> GSHMASMKKKGSVVIVGRINLSGDTAYAQQTRGEEGCQETSQTGRDKN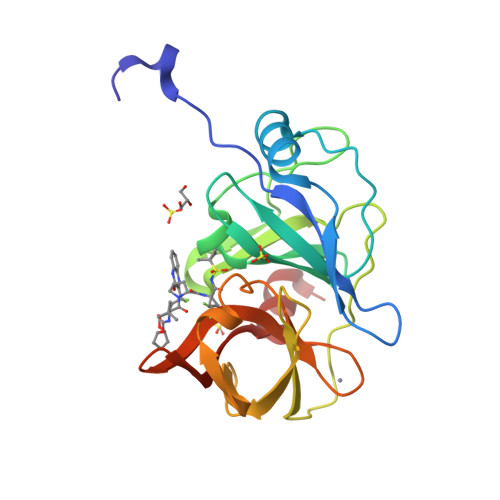QVEGEVQIVSTATQTFLATSINGVLWTVYHGAGTRTIASPKGPVTQMYTNVDKDLVGWQAPQGSRSLTPCTCGSSDLYLVTRHADVIPVRRRGDSRGSLLSPRPISYLKGSSGGPLLCPAGHAVGIFRTAVCTRGVAKAVEFIPVESLETTMRSP> SFSGVVDIIVVRQPDDSLKSMPFHIRFGTLKVLDNQNINIQITVNDKKIEDVFMLMLPEGACYFPELNAKNEIQKKLRPSSAILKKFNLKNGYNKIQFIAESDLQGKQLIEGKIYLYNYDTKLVISDVNGTVTKSDVKGH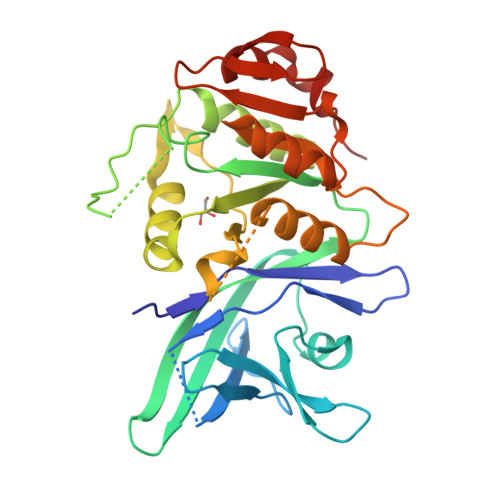ISTIIGKEWTHDDIAELYTNIQKNGYKMVYLSSRPLYFYNYTQGYLKGIIQNGFTMPDGPILLSPDQIISSLNREVVYKKADEFKGALLKDLRRVFPEEVNPIFAGFGNRDTDATACLYAGVIIDNIFIINEQSQVEILGKQEKSSYKKINEKIQELFPRLP>[3x]ALGDTLTITLG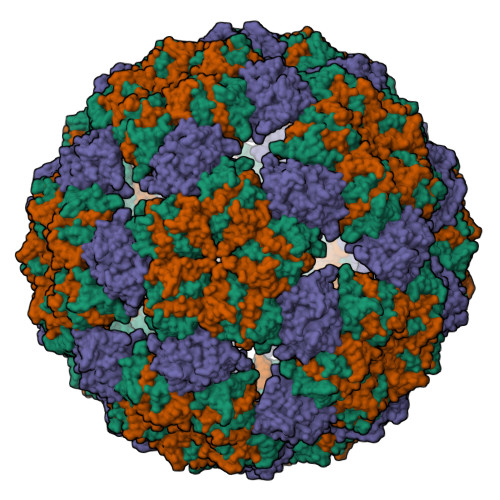GSGGTAKVLRKINQDGYTSEYYLPETSSSFRAKVRHTKESVKPNQVQYERHNVEFTETVYASGSTPEFVRQAYVVIRHKVGDVSATVSDLGEALSFYLNEALYGKLIGWES> GSPSTRDYEIQRERIELGRCIGEGQFGDVHQGIYMSPENPALAVAIKTCKNCTSDSVRE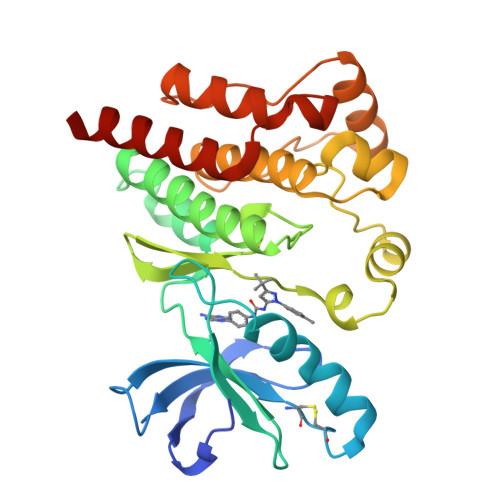KFLQEALTMRQFDHPHIVKLIGVITENPVWIIMELCTLGELRSFLQVRKYSLDLASLILYAYQLSTALAYLESKRFVHRDIAARNVLVSSNDCVKLGDFGLSRYMEDSTYYKASKGKLPIKWMAPESINFRRFTSASDVWMFGVCMWEILMHGVKPFQGVKNNDVIGRIENGERLPMPPNCPPTLYSLMTKCWAYDPSRRPRFTELKAQLSTILEEEKAQ N,N'-(ethane-1,2-diyldibenzene-3,1-diyl)dithiophene-2-carboximidamide | C24 H22 N4 S2 | 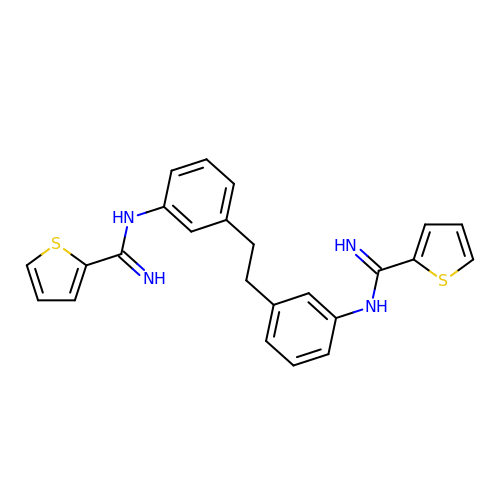MNMWXAHXXVXJBB-UHFFFAOYSA-N>[4x]MSFPGWGPYPPVERDETSAITYSSKLHGSVTVRDPYSQLEVPFEDSEETKAFVHSQRKFARTYLDENPDREAWLETLKKSWNYRRFSALKPESDGHYYFEYNDGLQSQLSLYRVRMGEEDTVLTESGPGGELFFNPNLLSLDGNAALTGFVMSPCGNYWAYGVSEHGSDWMSIYVRKTSSPHLPSQERGKDPGRMNDKIRHVRFFIVSWTSDSKGFFYSRYPPEDDEGKGNAPAMNCMVYYHRIGEDQESDVLVHEDPEHPFWISSVQLTPSGRYILFAASRDASHTQLVKIADLHENDIGTNMKWKNLHDPWEARFTIVGDEGSKIYFMTNLKAKNYKVATFDANHPDEGLTTLIAEDPNAFLVSASIHAQDKLLLVYLRNASHEIHIRDLTTGKPLGRIFEDLLGQFMVSGRRQDNDIFVLFSSFLSPGTVYRYTFGEEKGYRSLFRAISIPGLNLDDFMTESVFYPSKDGTSVHMFITRPKDVLLDGTSPVLQYGYGGFSLAMLPTFSLSTLLFCKIYRAIYAIPNIRGGSEYGESWHREGMLDKKQNVFDDFNAATEWLIANKYASKDRIAIRGGANGGVLTTACANQAPGLYRCVITIEGIIDMLRFPKFTFGASWRSEYGDPEDPEDFDFIFKYSPYHNIPPPGDTVMPAMLFFTAAYDDRVSPLHTFKHVAALQHNFPKGPNPCLMRIDLNSGHFAGKSTQEMLEETADEYSFIGKSMGLTMQTQGSVDSSRWSCVTV;>GFPWVIVVGVIGVIG[4x]

OphP is an essential enzyme for the biosynthesis of the macrocyclic peptide natural product omphalotin A. The enzyme has been proposed to proteolytically release a peptide intermediate from the precursor protein OphMA and to macrocyclize the multiply α-N-methylated core of this intermediate to produce omphalotin A. Our *in vitro* experiments demonstrate that OphP does not process OphMA but shows robust macrocyclase activity on pre-processed α-N-methylated peptides. OphP tolerates sequence promiscuity in the substrate but has a preference for highly α-N-methylated substrates and for N-methylated glycine residue at the catalytic site. The promiscuity of OphP is explained by structural analysis of co-complexes which reveals a predominantly hydrophobic substrate binding cleft with few interactions between substrate side chains and OphP. Similar to other POPs, the monomer has two domains, an α/β hydrolase domain (residues 1–82, 453–738) and the seven-bladed β-propeller domain (residues 83–452) ([Fig fig4]).

To characterize the interactions of OphP with its presumed natural substrate, S580A mutant crystals were soaked with a ten-fold methylated Oph-18mer^NL^ (W1-^me^V2-I3-^me^V4-^me^V5-^me^G6-^me^V7-^me^I8-^me^G9-V10-^me^I11-^me^G12-S13-^me^V14-M15-S16-T17-E18) and a seven-fold methylated Oph-15mer substrate (G1-F2-P3-W4-^me^V5-I6-^me^V7-^me^V8-^me^G9-^me^V10-^me^I11-^me^G12-V13-I14-G15) ([Fig fig2]) (both substrates yield dodecameric macrocycles with the underlined residues). The Oph-18mer^NL^ complex was obtained at 2.0 and the Oph-15mer complex at 2.5 Å resolution. In the Oph-15mer complex, residues G1-F2-P3-W4-^me^V5-I6-^me^V7-^me^V8-^me^G9-^me^V10-^me^I11 were located in the electron density in subunit D ([Fig fig4]) but there is evidence of disorder in the peptide. The two complexes overlay with an RMSD of 0.9 Å over 719 residues. In contrast to the Oph-18mer^NL^ complex structure, residue ^me^G12 which is attacked by Ser580 to generate the macrocycle is not at the P1 pocket ([Fig fig4]). Rather the peptide bond of ^me^V8 is closest to this residue ([Fig fig4]). The peptide adopts a different conformation in the active site and as a result, the side chains in this complex make different interactions than the 18mer^NL^ ([Fig fig4]**)**. The substrate is not aligned properly for catalysis as the carbonyl of ^me^Val8 is tilted and no longer hydrogen bonds to the canonical oxyanion hole. The side chain of ^me^V8 contacts Ile606 and Trp621 in the hydrophobic P1 pocket identified in the 18mer^NL^ complex. **(**[Fig fig4]**)**. This complex demonstrates the plasticity of peptide recognition by OphP – rather than disclosing additional mechanistic insights – and perhaps explains its rather broad substrate specificity, as there don’t seem to be clearly specific interactions with the substrate except for the P1 pocket residue.> HHHHHHEGFIEDASVSLGLRNLYFNRDFRQPGAAQSKQEEWAQGFLLQAKS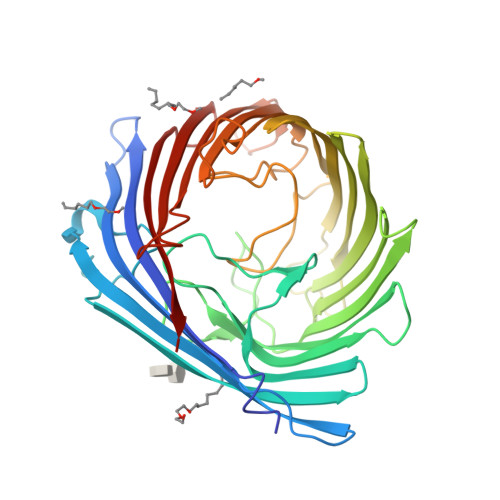GYTQGTLGLGVELIGQLGLKLDSSPDRAGSGLLPRHADGRAADDYARLGVAPKLKLSNTELKLGELLPELPILLRNDGRLLPQTFQGGMLTSREIAGLTLHGGQMRSLSQRNSSDHQDLSVDGRGGAFSDRFDYLGAEYRFNAERSQVGLWQARLQDIYRQDYYSLSHKQSFGGWRLGASVGLFDTRDEGAAKLGELENRALTGFFSATRGGHSLGAGYQRMYGDDGMLYIAGTSTPLVNDIQVRNFTSAGERSWQLRYDYDFVALGIPGLTAMARYASGAHARTKAMDDGRAWERDVDVAYVIQSGPLKNLGLRWRNAMLRSNHAADVDENRLILSYSLPLL>[2x]MSTFEDADTEETVTCLQMTIYHPGQQSGIFKSIRFSSKEKFPSIEVVKFGRNSNMCQYTFQDKQVSRIQFVLQPFKQFNSSVLSFEIKNMSKKTSLMVDNQELGY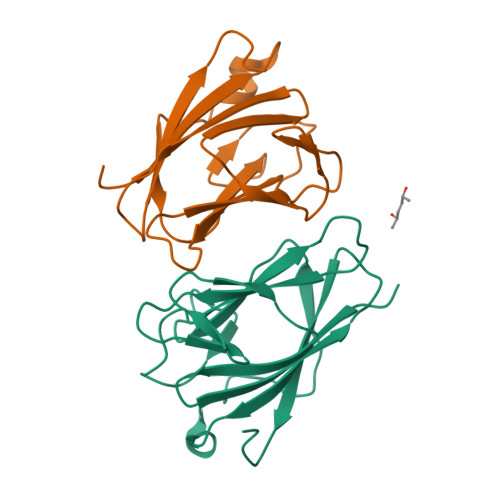LNKMDLPYKCMLRFGEYQFLLQKEDGESVESFETQFIMSSRPLLQ;>[2x]GPLGSMERPLTVLQVSLYHPTQGPVAFAHVPQQLQHDASRLLVGRGQNTHLQLQLPQLSRYHLSLEPYLEKGSSLLAFCLKVLTRKSCVWVNGLPLRYLEQVPLGTINRISFSGIQMLVRKEGGASLETFVCYFHLSPSPLIYR>SNAMARGVNKVILIGNLGQDPEVR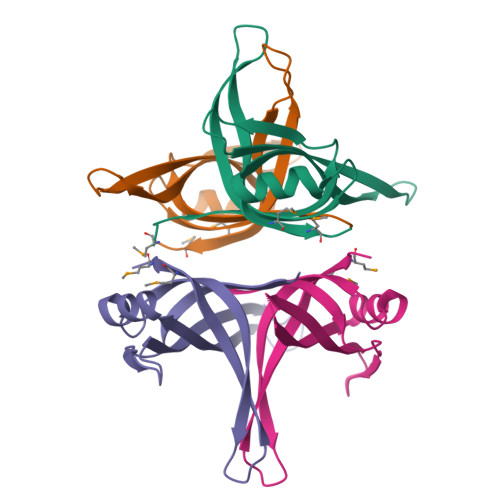YTPNGNAVANVTLATSTTWRDKQTGELQERTEWHRIAFFNRLAEIVGEYLRKGSKIYIEGSLRTRKWQDKNGVDRYTTEIIANEMHMLDNRGGGNSGNYGNHSEGGASNKQSAPTSSQTPTAGDDSSVADFDDD[4x]> MLKQVEIFTDGSCLGNPGPGGYGAILRYRGREKTFSAGYTRTTNNRMELMAVIVALEALKEHCEVILSTDSQYVRQGITQWIHNWKKRGWKTADKKPVKNVDLWQRLDAALGQHQIKWEWVKGHAGH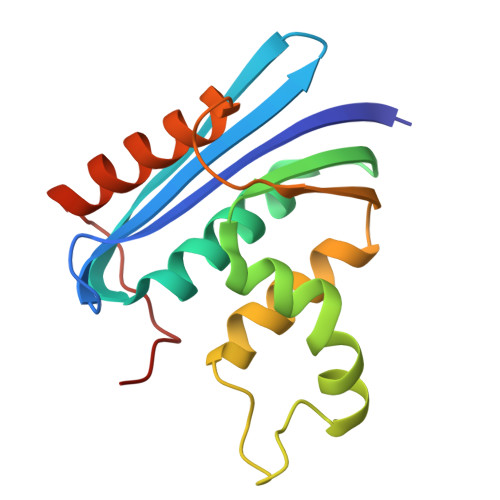PENERCDELARAAAMNPTLEDTGYQVEV> TRATNDERCKILEQRLEQGMVFTEYERILKKRLVDGECSTARLPENAERNRFQDVLPYDDVRVELVPTKENNTGYINASHIKVSVSGIEWDYIATQGPLQNTCQDFWQMVWEQGIAIIAMVTAEEEGGREKSFRYWPRLGSRHNTVTYGRFKITTRFRTDSGCYATTGLKMKHLLTGQERTVWHLQYTDWPEHGCPEDLKGFLSYLEEIQSVRRHTNSTSDPQSPNPPLLVHSSAGVGRTGVVILSEIMIACLEHNEVLDIPRVLDMLRQQRMMLVQTLCQYTFVYRVLIQFLKSSRLI

PTPN21 belongs to the four-point-one, ezrin, radixin, moesin (FERM) domain–containing protein tyrosine phosphatases (PTP) and plays important roles in cytoskeleton-associated cellular processes like cell adhesion, motility, and cargo transport. Because of the presence of a WPE loop instead of a WPD loop in the phosphatase domain, it is often considered to lack phosphatase activity. However, many of PTPN21’s biological functions require its catalytic activity. Combined with biochemical analysis, we have found that PTPN21 PTP is weakly active and is autoinhibited by association with its FERM domain.

To further investigate the working mechanism of the phosphatase domain of PTPN21, we determined structures of PTPPTPN21 C1108S in complex with a phosphate ion as well as PTPPTPN21 C1108S in complex with a Src pY530 peptide. In the 2.0-Å PTPPTPN21 C1108S structure with a phosphate ion in the active site, the electron density of the phosphate ion and two nearby water molecules is well defined. The phosphate group is 3.3 Å from the hydroxyl group of S1108, and the oxygen atoms of the phosphate group hydrogen bond to main chain amides in the P loop. The scissile oxygen forms two hydrogen bonds with two water molecules, one of which is the “catalytic water” (WA1). The water molecules themselves are coordinated by Q1152 and Q1156 in the Q loop as well as E1067 in the WPE loop. The carboxyl group of E1067 is close to the scissile oxygen with a distance of 2.7 Å. Compared to the PTPPTP1B-pY complex, water molecule 2 (WA2) occupies the position of the tyrosine moiety, and Q1152 is in a downward conformation due to the absence of tyrosine. It is likely that WA2 and E1067 as well as WA1 serve to stabilize the phosphocysteine intermediate after P─O bond breakage, and what we captured in Fig. 3B is a product-complex conformation. The invariant R1114 residue is held in place by electrostatic interactions with the inorganic phosphate and E1001. In addition, R1114 forms a hydrogen bond with the backbone carbonyl group of W1065, which helps to maintain the WPD loop in the closed conformation. Close examination of the electron density revealed that C1155-C1070 in the open structure formed a disulfide bond, while C1155 and C1070 in the WPE closed structure are free with a distance around 3.9 Å.Calcium homeostasis modulators (CALHMs/CLHMs) comprise a family of pore‐forming protein complexes assembling into voltage‐gated, Ca2+‐sensitive, nonselective channels. These complexes contain an ion‐conduction pore sufficiently wide to permit the passing of ATP molecules serving as neurotransmitters. C. elegans expresses only a single homolog of CALHM1, termed CeCLHM1, in its sensory neurons and muscle cells. In these cells, CeCLHM1 forms a Ca2+‐sensitive ion channel involved in regulating the function of excitable cells and maintaining normal motility of the worms.

Here, we present the structure of the Caenorhabditis elegans CLHM1 channel in its open state solved through single‐particle cryo‐electron microscopy at 3.7‐Å resolution. The transmembrane region of the channel structure of the dominant class shows an assembly of 10‐fold rotational symmetry in one layer, and its cytoplasmic region is involved in additional twofold symmetrical packing in a tail‐to‐tail manner. the doubled‐layered channel of CeCLHM1 is formed by docking the C‐terminal domains (CTDs) from two decameric hemichannels in a tail‐to‐tail manner. The double‐layered 20‐mer channel spans ~170 Å in length along the direction of the membrane normal, and is ~130 Å in width. The channel contains a wide funnel‐like pore with a diameter of approximately 40 Å around the narrowest central region, and over 60 Å around the extracellular and intracellular entrance. Thus, the structural model of CeCLHM1 represents an open‐state form of the channel, as any other structural adjustment would probably further constrict the pore size. Each of the 20 identical protomer subunits shows an L‐shaped structure. A bundle of five TM helices and a long cytoplasmic helix form the vertical and horizontal arms, respectively. S2–S4 helices span the membrane and form the outer wall of the channel, whereas both S0 and S1 line the interior of the channel and are about one to three helix‐turns shorter at both ends. S0 and S1 are tightly packed against the outer wall, shaping a widely open pore at the central region of the channel, and the lumen surface of the pore exhibits alternating layers of positive and negative charges.

>MTTSINSVVTVFQNVFTNHGSTLLNGILIATTVGGQSLVRKLTFSCPCAYPLNIYHSLVFMFGPTAALLLIGITVNSTTWKLAHGFFFRVRDTRHSWKTTCVSWIEVLIQSSVAPIAWLFVVFLDGGYYRCYRSHEFCLISDAILCKNSTILNSYASTSSFNKISDNGKYCPPCICVPNPTDASYLEAESQIYAWGLLLFSGVAAFLVITCNRMCDKYTLVQRQYVETYKNVETQKFDAVAKEHASQLAEHNARAFFGQKDWTKRDWDWVSGIPEVNNPLFARLRLIAAEKTQQTMYTPLQLWNDNKGYRIPQPDLQLTQIIVDETKED[20x]One such system is the PreQ1 riboswitch, which binds to the small, modified nucleotide 7-aminomethyl-7-deazaguanine (known as PreQ1). Upon recognition of PreQ1, the RNA changes conformation and alters gene expression at either transcriptional level or translational level. For the PreQ1 riboswitch from Thermoanaerobacter tengcongensis (Tt-preQ1-RS) binding to PreQ1 also results in the formation of an H-type pseudoknot structure. However, in this case the riboswitch acts at the translational level by regulating the accessibility of the Shine-Dalgarno sequence and ribosome binding.

To further validate the binding of 11 to the PreQ1 aptamer, we performed X-ray crystallography with the PreQ1 aptamer from T. tengcongensis (Tt-preQ1-RS), using a previously reported method. Co-crystals were obtained using wild type (WT) and an abasic mutant at positions 13 and 14 (ab_13-14) without photocrosslinking, and the complex structures were solved by the molecular replacement method at 2.80 and 1.57 Å resolution respectively. Positions A13 and A14 of the Tt-preQ1-RS are important for stabilization of the expression platform. However, when we co-crystallized the wild-type Tt-preQ1-RS with the compound 11, only small co-crystals were obtained that diffracted to 2.8 Å resolution. Importantly, the binding mode of the compound is conserved between the WT and abasic mutant crystals and the RNA structures are quite similar with the exception of the nucleotides from positions 12 to 14. No specific interaction is observed between the alkyne handle and the RNA, suggesting that positions 12 to 14 are not involved in the direct interaction for binding of the compound 11. An X-ray co-crystal structure of the probe in complex with the aptamer demonstrated that the mode of binding was unperturbed by the introduction of the crosslinker sidechain.

> CUGGGUCGCAGUAACCCCAGUUAACAAAACAAG> MDDISVIKNEDYEGSHRFLAEELLMPNANKTDGNRSTMFCSHLAQAVTLQKAEPPLVYTNFENQVGKYSTAGYRKANSNYKVIEKIYKNDYNYVLIVQDQETGEYTLFERAECEFLTEHYGFQWDNDKIDSLKKDDTIEKDTVLYKNTCYDENMNFGYGVNLNAAYFSYKNETLEDAIVISESAAKKLGTFSVNKVKVSVNTNDILLNLYGDNENYKGFPDIGEHIKNQIIASRRRFDYNTALYELKNLNEMRDSDTPFFADGKIVDIEIFSNVPEEELKVQKYNEQVLYYINKQKEFSNNVYQKLKKIVEGKDNNVSDKLLHFYNNCKMRIDENISYTYQNSKFSGFIMEFTILEEEPLNKGSKITGRYGNKGVISKILPDDQMPTVAEGRFKGLKADICLNPLGVFNRLNPSQLIEQELNWIAKFIRKDMEEAGSNEEKV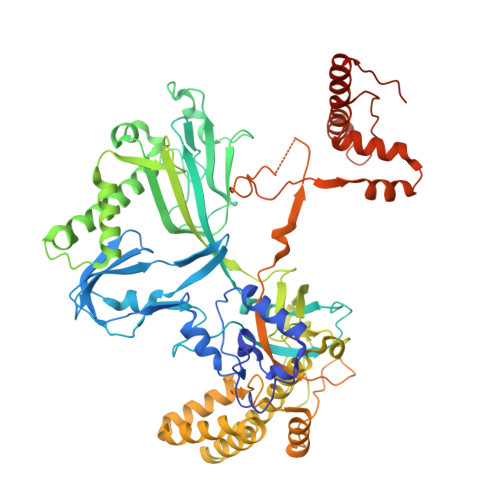SILLDFLNRVNKEETELMEEFINSLNKTELEEFLNDIIENGIPICQKPFFGNIGLDELWELYNHYDHIDYFKCEGISTPLIIGEIYMVRLKHEPHSKFSARSTSFMNLRGLPAKSKNFKEHKDLYSKTPVRIGNMEISNLSLTNEMGSIMDMLNSYSNNETNRRELIMQLLTGNPFDTNIDLSDVESGTSKILKSLFTCLGLSIDDVEEEWENKLNGKVEDEK> MIFSVDKVRADFPVLSREVNGLPLAYLDSAASAQKPSQVIDAEAEFYRHGYAAVHRGIHTLSAQATEKMENVRKRASLFINARSAEELVFVRGTTEGIDLVANSWGNSNVRAGDNIIISQMEHHANIVPWQMLCARVGAELR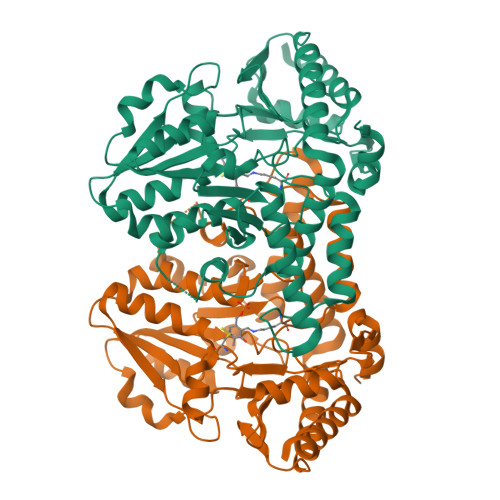VIPLNPDGTLQLETLPTLFDEKTRLLAITHVSNVLGTENPLAEMITLAHQHGAKVLVDGAQAVMHHPVDVQALDCDFYVFSGHKLYGPTGIGILYVKEALLQEMPPWEGGGSMIATVSLSEGTTWTKAPWRFEAGTPNTGGIIGLGAALEYVSALGLNNIAEYEQNLMHYALSQLESVPDLTLYGPQNRLGVIAFNLGKHHAYDVGSFLDNYGIAVRTGHHCAMPLMAYYNVPAMCRASLAMYNTHEEVDRLVTGLQRIHRLLG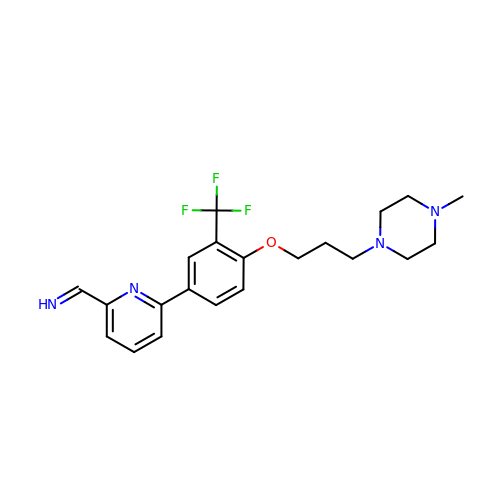(E)-1-(6-{4-[3-(4-methylpiperazin-1-yl)propoxy]-3-(trifluoromethyl)phenyl}pyridin-2-yl)methanimine | C21 H25 F3 N4 O | BNDJQLLXZUKTHM-MFKUBSTISA-N>MSSKYAVKLKTDFDNPRWIKRHKHMFDFLDINGNGKITLDEIVSKASDDICAKLEATPEQTKRHQVCVEAFFRGCGMEYGKEIAFPQFLDGWKQLATSELKKWAR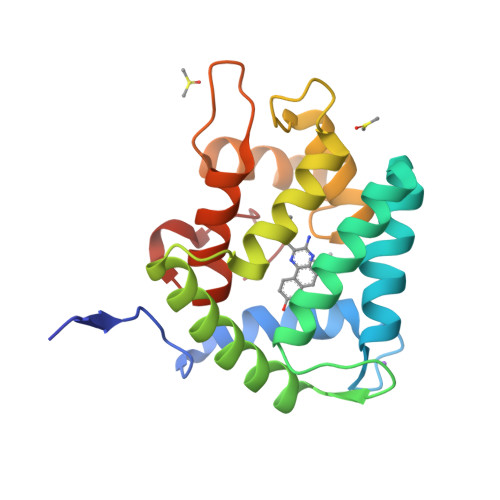NEPTLIREWGDAVFDIFDKDGSGTITLDEWKAYGKISGISPSQEDCEATFRHCDLDNSGDLDVDEMTRQHLGFWYTLDPEADGLYGNGVP[2x]> ELSTSLYKKAGFHHHHHHENLYFQDSNTKGWSEVLKGSECKPRPIVVPVSETHPELTSQRFNPPCVTLMRCGGCCNDESLECVPTEEVNVTMELLGASGSGSNGMQRLSFVEHKKCDCRPRFTTTPPTTTRPPRRRR;> HQHGVVYITENKNKTVVIPCLGSISNLNVSLCARYPEKRFVPDGNRISWDSKKGFTIPSYMISYAGMVFCEAKINDESYQSIMYIVVVVGYRIYDVVLSPSHGIELSVGEKLVLNCTARTELNVGIDFNWEYPSSKHQHKKLVNRDLKTQSGSEMKKFLSTLTIDGVTRSDQGLYTCAASSGLMTKKNSTFVRVHEKPFVAFGSGMESLVEATVGERVRIPAKYLGYPPPEIKWYKNGIPLESNHTIKAGHVLTIMEVSER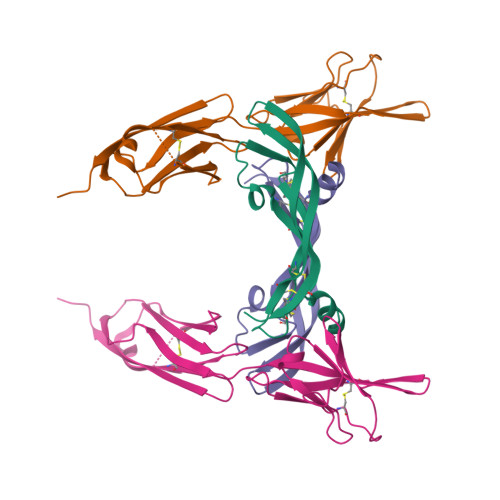DTGNYTVILTNPISKEKQSHVVSLVVYVPPQIGEKSLISPVDSYQYGTTQTLTCTVYAIPPPHHIHWYWQLEEECANEPSQAVSVTNPYPCEEWRSVEDFQGGNKIEVNKNQFALIEGKNKTVSTLVIQAANVSALYKCEAVNKVGRGERVISFHRTHHHHHH> MPEKKIDGRRKA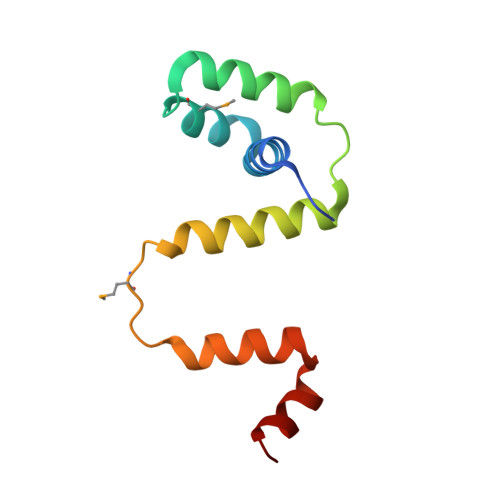AVLLVALGPEKAAQVMKHLDEETVEQLVVEIANIGRVTPEEKKQVLEEFLSLAKAKEMISEGGIEYAKKVLEKAFGPERARKIIER>[2x]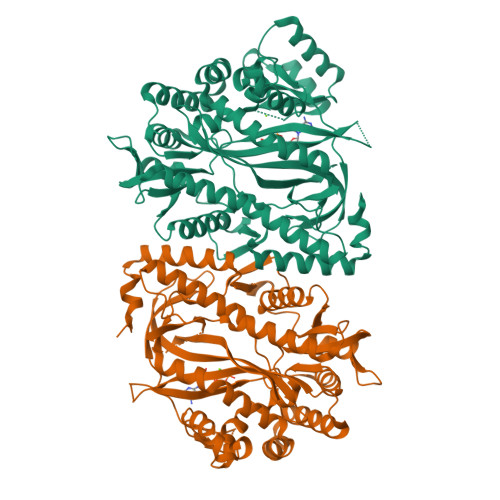MNCDNAKFIIFFFFIIFLCANFAVCNELEDYVEKSVNSETKLHKLADFAIDWAHNNGLILRTKQFLNKSDVAEFAPVSLLPSPFPRHAFEKAVAVHEALQLLYFRVACDYEFMMDAYKDVVNTDNHLRQLVNIIKDAHKQGIKQPTTLLIMRADYMLNTLNSKGNDDEYELKQVEVNTGAIGGLGIDRRTTELHRQMLRKVGMDTSNSPANNGDSNMIESLFMAWEAFGNKNALFVFLSHERLQYKFELRNIQCQLEELSNGQMKVEYVSLKAGYEQLKLGEDYSLLLNGEIVGVVYSTISALGHQANAREMEARRTIELSNAIKAPSLAIAISSSKKIQQLLTTPGTLERFFPSATEADKVAAIRETFTGLWGLEKSDDQTERRIKDAIENPANYVLKSNGECGGNNFYDEALAEKLRTMPQAERASHILMQKLIPMATKNYFLRPFHEPKLNVVVGELGVNGTLLGNLRDQSVRHNVQSGHLLRTKLREANEGGISVGTGVGDSPYLF> GVENAEKGVTENTDATADFVAQPVYLPENQTKVAFFYDRSSPIGRFAVKSGSLESGFAPFSNKACPNSVILTPGPQFDPAYD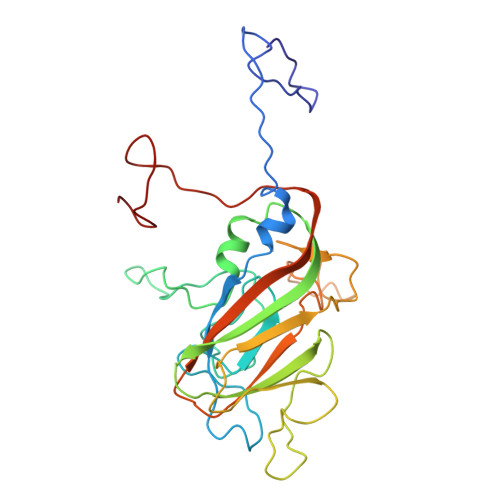QLRPQRLTEIWGNGNEETSEVFPLKTKQDYSFCLFSPFVYYKCDLEVTLSPHTSGAHGLLVRWCPTGTPTKPTTQVLHEVSSLSEGRTPQVYSAGPGTSNQISFVVPYNSPLSVLPAVWYNGHKRFDNTGDLGIAPNSDFGTLFFAGTKPDIKFTVYLRYKNMRVFCPRPTVFFPWPTSGDKIDMTPRAGVL> MSGVRAVRISIESACEKQVQEVGLDGTETYLQPLSMSQNLARLAQRIDFSQGSGSEEEEAAGPDGDAPDWGGAGADQDDEEGLVKFQPSLWPWDSVRNNLRSALTEMCVLYDVLSIVRDKKFMTLDPVSQDALPPKQSPQTLQLISKKKSLAGAAQILLKGAERLTKSVAENQENKLQRDFNSELLRLRQHWKLRKVGDKILGDLSYRSAGSLFPHHGTFEVIKNTDIDLDKKIPEDYCPLDVQIPSDLEGSAYIKVSIQKQAPDIGDLGTVNLFKRPLPKSKPGSPHWQTKLEAAQNVLLCKEIFAQLSREAVQIKSQIPHIVVKNQIISQPFPSLQLSISLCHSSDDKKSQKCAAEKPGQEDHLYVLEHNLHLLIREFHKQTLSSIVMPHPASAPFGHKRMRLSGPQAFDKNEINSIQSTEGLLEKIIKQAKHIFLRSRTAATIDSLASRIEDPQIQAHWSNINDVYESSVKVLITSQGYEQICKSIQLQLNIGVEQVRVVHRDGRVIMLSHQEQELQDFLLSQMSQHQVHAVQQLAKVMGW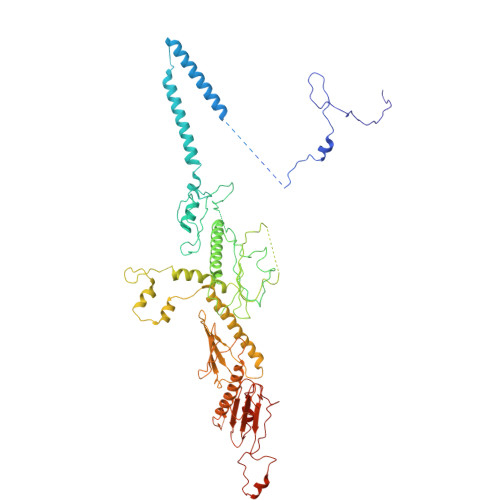QVLSFSNHVGLGPIESIGNASAITVASPSGDYAISVRNGPESGSKIMVQFPRNQCKDLPKSDVLQDSKWSHLRGPFKEVQWNKMEGRNFVYKMELLMSALSPCLL> TK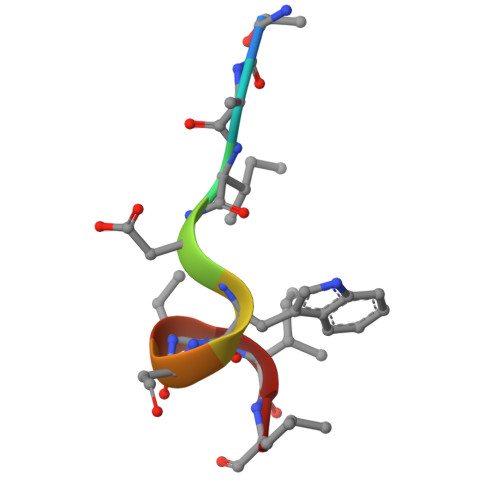IDWNKIL The Rnf complex is the primary respiratory enzyme of several anaerobic prokaryotes that transfers electrons from ferredoxin to NAD+ and pumps ions (Na+ or H+) across a membrane, powering ATP synthesis. The complex comprises six subunits, with three integral membrane subunits RnfA/D/E, two membrane-anchored proteins RnfB and RnfG, and an attached cytoplasmic protein, RnfC. On the cytoplasmic side, the complex comprises RnfC and RnfB that are responsible for the interactions with the soluble electron carriers, whilst the periplasmic side harbours the flavoprotein RnfG. We show that the reduction of the unique membrane-embedded [2Fe2S] cluster electrostatically attracts Na+, and in turn, triggers an inward/outward transition with alternating membrane access driving the Na+ pump and the reduction of NAD+.

We obtained two structural snapshots of the Rnf complex that represent states along the reverse and direct electron transfer directions during catalytic turnover conditions: (1) an NADH-reduced state resolved at 3.3 Å resolution, and (2) a Fd-reduced state at 2.8 Å resolution, with the Fd purified from Clostridium pasteurianum and reduced by catalytic amounts of a CO dehydrogenase obtained from A. woodii. Since all determined structures have overall the same organisation and cofactor content, we focused our description on the Rnf complex with the bound NADH. The NADH-binding RnfC subunit is the only subunit that is not membrane-bound. RnfC has a globular flavin-binding domain and a small helical C-terminal domain that binds two [4Fe4S] clusters (C1 and C2), with similarities to the FMN site of respiratory Complex I (Nqo1) and HydABC (HydB). In the determined structure, we observed a well-resolved density for a bound NADH molecule, which forms stacking interactions to the non-covalently bound FMN cofactor. In addition, unstructured N- and C-terminal loops of RnfD bind to the cavities within RnfC that stabilise the subunit and could be partially resolved in our cryo-EM data. In RnfC, all cofactors are linearly arranged to the polytopic membrane protein RnfD and located at distances that could enable an efficient electron transfer across the complex. In simulations initiated from the NADH-reduced structure, the RnfA/E dimer samples an extracellular/periplasmic open (outward-facing) conformation.

> MTLIFIMISAIFVNNFVLSRFLGICPFLGVSKQVETAVGMGVAVTFVMALASAITYVVQYAILDPLSLGYLQTIAFILIIAALVQLVEMIIKKSSPSLYQALGVYLPLITTNCAVLGVALINIQNEYNFIETIFNGVGAALGFTLAIVLFAGIRERLETSAVPKALEGFPIALLTAGLMAIAFLGFSGMKL;> MLNAILVPVGILGVFGLIFGIGLAIAAKVFEVYEDPRVPLVRAALPGANCGGCGLPGCDALAANIVGGSAAIDACPVGGASCAAAVAEIMGMEAGSAVKKVATVICQGTCETAPNRAEYYGEMDCREAMIASGGSKGCRYGCLGYGTCKAVCPFDAIVIGEDGLPKVDPEKCTSCGKCVEACPKSIMTLVPEAQEVIVKCHNFDKGKIARLSCTTACIACGACVKACRFDAITVENNCAKIDYDKCRQCYECVDKCPMNCISGDVEYGKSTAYIIEENCIACGLCAKNCPVNAITGEIKKPPYVIDHDMCIGCGICFDKCRKSAIEMRPNKTK;> MNVKHGTFKGGIHPPYRKESTAEVPLGFGKKPEMVIIPMSLHIGAPCTPIVKKGDTVFLGQRVGEPNGFVSVPVHASVSGKVIAVEERPHASGDRVMSVVIESDGLDTIDPSIKPYGTLEDMDADAIKKMVLNAGIVGLGGATFPTHVKLAIPPDKKVDCVVLNGAECEPYLTADHHLMTSQAEKVVMGLKLAMKSVGVEKGFIGVEDNKTDAIEALVKAIGNDSRLEVYSLHTKYPQGAEKQLIAAITGREVPSGALPADAGVVVMNVGTAAQIAESMITGLPLYKRYLTCTGDAIKNPQTIEIRIGVPFQSVIDQCGGFSSEPGKVISGGPMMGVTQFVTDIPVMKGTSGILCLTKESAKIATPSNCIHCGKCVGVCPIHLQPLNIAEYSQRNMWDKCESNNAMDCIECGSCSYICPAKRTLVSSIRVAKREIIAQRRKGN;> MNELNLTVSSSPHIRAKHSTASIMQNVIIALLPALAVAGYVFGLWALALVAICVISSVATEAVIQKLLKKPITVNDWSAVVTGVLLAFNLPINAPWWIGVVGSVFAIAIVKQCFGGLGQNFINPALAARAFLLASWPGHMTSTAYIPLTDTVTTATPLALLKAGETGSMPSTLDLFTGLNGVYGCIGEISALALLIGGLYLIYKGIISWRIPTIYLLTIAIFALLVGQDPIVHMVSGGVMLGAFFMATDYASSPVTAKGQIIYAIGCGLITMIIRLYGGYPEGCSYSILLMNVATPLIERFTKERIYGVTKIKKEAKA;> MNFMKNLTRGIIRENPTFVLVLGMCPTLAVTTSAINGMGMGLATMLVLIGSNVAISALRKVIPDNIRIPAFVVVIASFVTIVGMLMKAYVPALDAALGIFIPLIVVNCIILARAEAFAFSNGIADSFADAVGMGLGFTLALTILGSIREILGAGSIFGFSLFGAAYEPVLLMILPPGAFLTLGLLIGLINWKTKKA;> METKEKVQIDWKVVFKLGLILFVISAVAACALALTNYVTAGTIEEMNVQTNTVARQEVLPKAADFEAVPAKDVEKIASEIGMEKPEELLEVYIGKSNGEVVGYTVKTGPTSGYAGEVQVLTGISADGVITGITIIKSNETPGLGAKASGVWNDQFTGKSAKEELVVVKGTTKEGSNEIQAITGSTITSKAVTSGVNMSIQVYQNLSK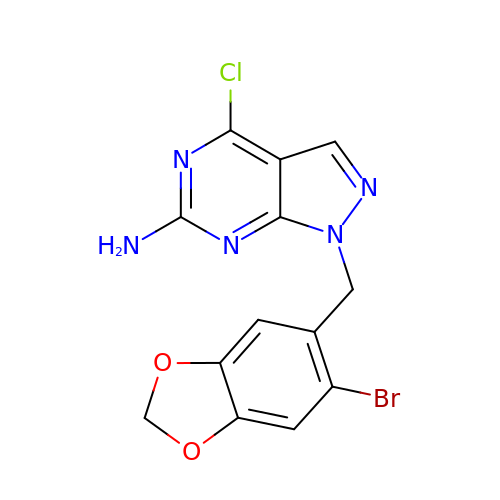1-[(6-bromanyl-1,3-benzodioxol-5-yl)methyl]-4-chloranyl-pyrazolo[3,4-d]pyrimidin-6-amine | C13 H9 Br Cl N5 O2 | BIABSXPPEYWVER-UHFFFAOYSA-N> SEICPSFQRVIETLLMDTPSSYEAAMELFSPDQDMREAGAQLKKLVDTLPQKPRESIIKLMEKIAQSSLSGCNSNVLSWQTYSWYCGSPSFQRVIETL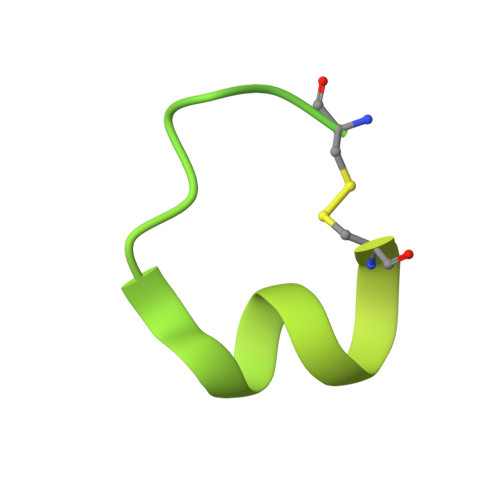LMDTPSSYEAAMELFSPDQDMREAGAQLKKLVDTLPQKPRESIIKLMEKIAQSSLCN>HHHHHHSSGLVPRGSHMMELLAKTRKLNALLQSAAGKPVNFREMSDTMCEVIEANVFVVSRRGKLLGYAIHQQIENERMKQMLAERQFPEEYTQSLFNITETSSNLDVNSAYTAFPVENRELFGQGLTTIVPIVGGGERL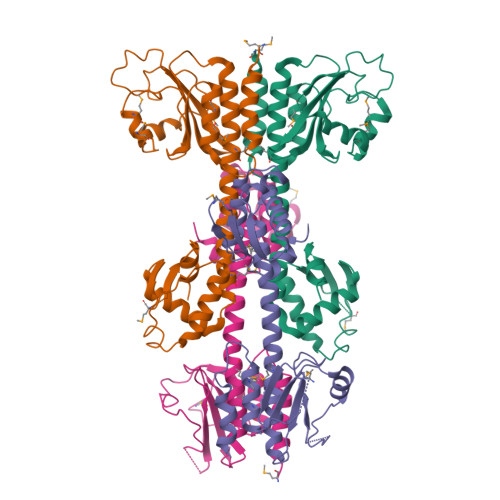GTLVLARLGQEFLDDDLILAEYSSTVVGMEILREKAEEIEEEARSKAVVQMAISSLSYSELEAIEHIFEELNGTEGLLVASKIADRVGITRSVIVNALRKLESAGVIESRSLGMKGTYIKVLNDKFLQELAKLKTN[4x]>PKEVIIHKNLSDALKTPNEVQILDLSRNQLTILPKEIEQLVNLESLHLRDNELTTLPEEIGILKNLKYLDISRNQISNFPKEIQKLKNLEVLFLNGNSLSN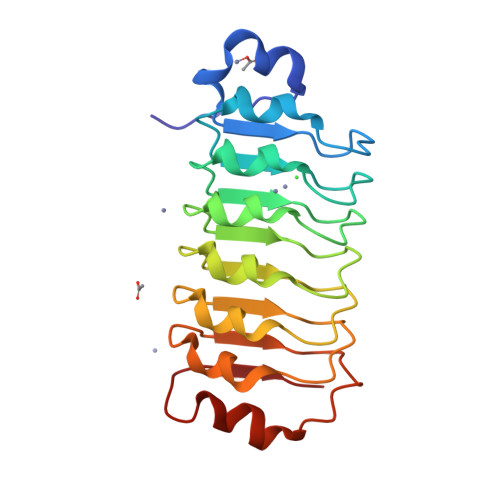LPEEIGELEKLGILYLNNNQLTTLPKEIGQLENLVSLSLSSNKLTSIPDELGQLKKLRILNLWDNPTLTTPERNIRKLFRNQEITIEIS[2x]> ETGKADRYKSHGKGYNWGNYNTETQKCEIFNVKPTCLINNAAYIATTALSHPIEVEGGGGSGGGGSGGGGSGGGGSNYMGNPWTEYMAKYDIEEVHGSGIRVDLGEDAEVAGTQYRLPSGKCPVFGKGIIIENSNTAFLTPVATGN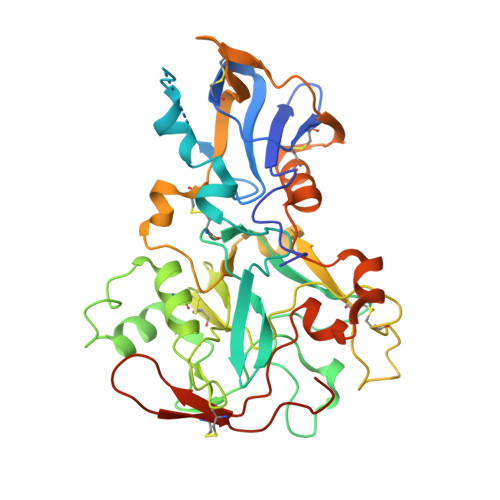QYLKDGGFAFPPTEPLMSPMTLDEMRHFYKDNKYVKNLDELTLCSRHAGNMIPDNDKNSNYKYPAVYDDKDKKCHILYIAAQENNGPRYCNKDESKRNSMFCFRPAKDISFQNYAYLSKNVVDNWEKVCPRKNLQNAKFGLWVDGNCEDIPHVNEFPAIDLFECNKLVFELSASDQPKQYEQHLTTQQAKDIGAGPVASCFTTRMSPPQQICLNSVVNTALSGTKHHHHHH>MSDKDSKNTPQVPEKLGLS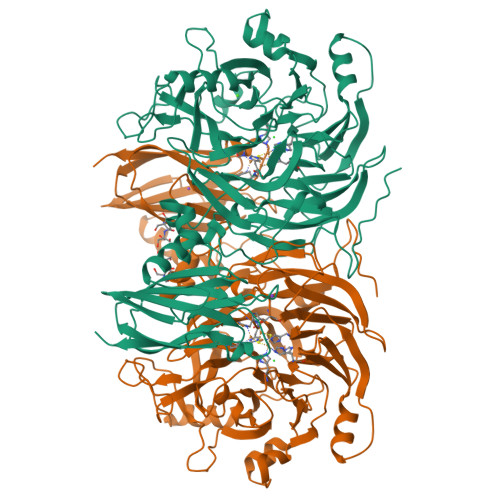RRGFLGASAVTGAAVAATALGGAVMTRESWAQAVKESKQKIHVGPGELDDYYGFWSGGHQGEVRVLGVPSMRELMRIPVFNVDSATGWGLTNESRHIMGDSAKFLNGDCHHPHISMTDGKYDGKYLFINDKANSRVARIRLDIMKCDKMITVPNVQAIHGLRLQKVPHTKYVFANAEFIIPHPNDGKVFDLQDENSYTMYNAIDAETMEMAFQVIVDGNLDNTDADYTGRFAAATCYNSEKAFDLGGMMRNERDWVVVFDIHAVEAAVKAGDFITLGDSKTPVLDGRKKDGKDSKFTRYVPVPKNPHGCNTSSDGKYFIAAGKLSPTCSMIAIDKLPDLFAGKLADPRDVIVGEPELGLGPLHTTFDGRGNAYTTLFIDSQVVKWNMEEAVRAYKGEKVNYIKQKLDVHYQPGHLHASLCETNEADGKWLVALSKFSKDRFLPVGPLHPENDQLIDISGDEMKLVHDGPTFAEPHDCIMARRDQIKTKKIWDRNDPFFAPTVEMAKKDGINLDTDNKVIRDGNKVRVYMTSMAPAFGVQEFTVKQGDEVTVTITNIDQIEDVSHGFVVVNHGVSMEISPQQTSSITFVADKPGLHWYYCSWFCHALHMEMVGRMMVEPA[4x]>[2x]ASMTGGQQMGRDQAGITGTWYNQLGSTFIVTAGADGALTGTYESAVGNAESRYVLTGRYDSAPATDGSGTA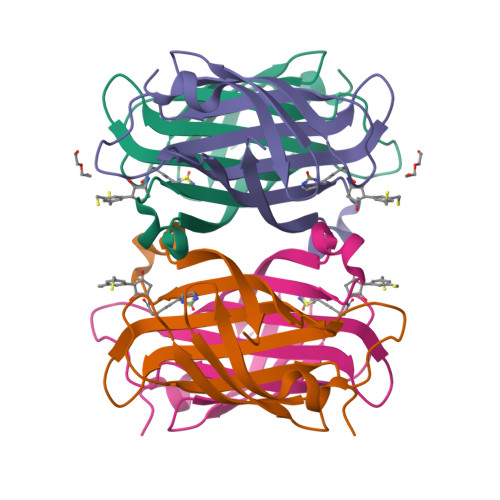LGWTVAWKNNYRNAHSATTWSGQYVGGAEARINTQWLLTAGTTEANAWASTLVGHDTFTKVKPSAASIDAAKKAGVNNGNPLDAVQQ> QAMLIGEIMDLNLKNFLEDREEIIRDAKRKDEKSFKDFKKIVEEIKERENKDKIVCDFTEYNPLHKGHKYALEKGKEHGIFISVLPGPLERSGRGIPYFLNRYIRAEMAIRAGADIVVEGPPMGIMGSGQYMRCLIKMFYSLGAEIIPRGYIPEKTMEKVIDCINKGYHIQVKPYKIICIETGEILGEKLNIDNYVIASMSQMIYKLNREGLKFNPKFVFVKRLEGISGTKIREAIFSGKFEDIKNMLPKTTLSILKELYDNGKLNE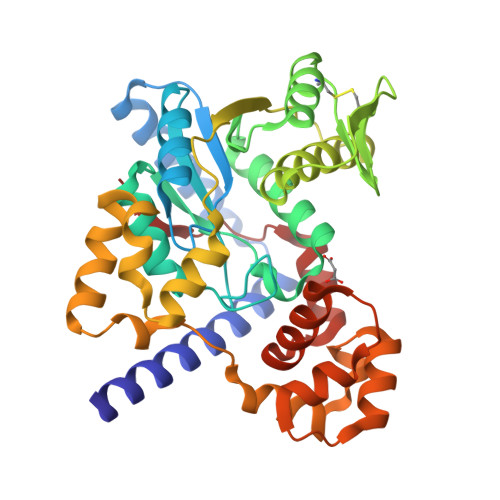LILKRFEDRILETANEYDLYEYLPSNVAEILEKKRPFNNIEEIKNSLPYGFSRHFRERILSKLEARIPNETLSKYINNYPAKIKILAVKL(1~{R},3~{S},5~{Z})-5-[(2~{E})-2-[(1~{R},3~{a}~{S},7~{a}~{R})-7~{a}-methyl-1-[(1~{S})-1-[(2~{S},5~{S})-5-(2-oxidanylpropan-2-yl)oxolan-2-yl]ethyl]-2,3,3~{a},5,6,7-hexahydro-1~{H}-inden-4-ylidene]ethylidene]-4-methylidene-cyclohexane-1,3-diol | C28 H44 O4 | 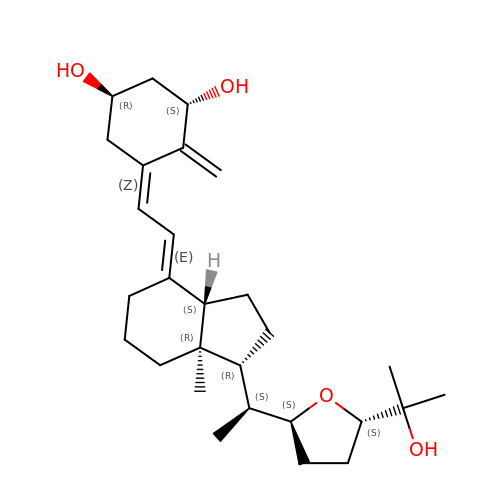DDIWZQGTNVZJGO-CWBZVJFYSA-N Recent work from our lab has shown that, in addition to classical FcR immunity mediated at the cell-surface, antibodies exert potent immune function from inside cells via a unique cytosolic IgG receptor called TRIM21. TRIM21 is a member of a large family of ~100 proteins with a common ‘tripartite motif’ architecture, comprising N-terminal RING, B-Box and coiled-coil domains. Instead of recruiting Src and Syk kinases, TRIM21 stimulates immune signaling via the activity of its RING domain, which catalyses the synthesis of polyubiquitin chains. Here we show that initiating ubiquitination is a key step in regulating TRIM21 activity and that a novel mechanism of autoinhibition and kinase-induced E2 enzyme recruitment controls its potent pro-inflammatory activity.

To understand how the B-Box modulates TRIM21 catalysis we solved a 2 Å crystal structure of the RING-Box protein. Surprisingly, this revealed that the B-Box occupies the E2 binding site on the RING domain. Comparison to the TRIM5α RING:E2 complex shows that the B-Box is located where helix 1 of the E2 would normally be positioned during RING binding. Crucially, the B-Box is able to occupy the E2 binding site on the RING by acting as an E2 mimic, forming similar electrostatic interactions. The RING surface contains a negatively charged patch, which is complementary to a strongly positively charged patch on both the E2 and the B-Box. In particular, Box-RING interaction is stabilized through a salt bridge between residues R118 and E12, which is analogous to the interaction between E2 residue R14 and RING residue E11 in the TRIM5:Ube2N structure. Taken together, these data suggest that the B-Box may be an autoinhibitory domain whose function is to regulate RING activity by preventing E2 recruitment. Moreover, the target serine in this motif is located at the centre of the B-Box:RING interface and undergoes phosphorylation in cells. The {1H}15N NOE ratios reveal that the most dynamic region is the linker (residues 83–102) between the RING and B-Box. This is in agreement with the higher temperature factors observed for these residues in the crystal structure.

>GSHMASAARLTMMWEEVTCPICLDPFVEPVSIECGHSFCQECISQVGKGGGSVCPVCRQRFLLKNLRPNRQLANMVNNLKEISQEAREGTQGERCAVHGERLHLFCEKDGKALCWVCAQSRKHRDHAMVPLE[2x]> KGSVV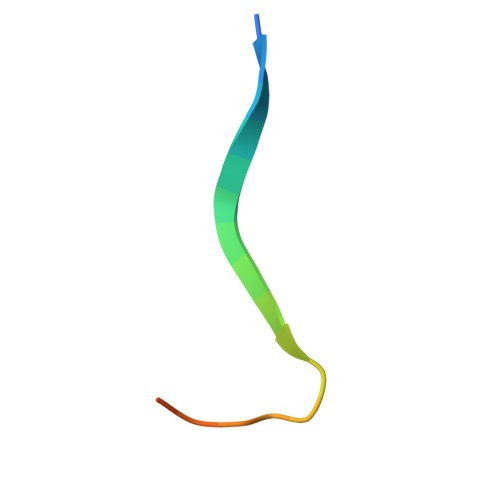IVGRIVLSGKPAIIPA p120RasGAP is a multidomain regulator of Ras signaling, containing two SH2 domains at its N-terminus and multiple other domains including a RasGAP. Binding of p190RhoGAP is mediated by phosphotyrosine-SH2 domain interactions, and a major driver is thought to be between the N-terminal SH2 of p120RasGAP and pTyr-1105 of p190RhoGAP. p190RhoGAP recruitment has multiple effects, including inhibition of Rho signaling by locating p190RhoGAP to the plasma membrane, and activation of Ras signaling by suppression of p120RasGAP’s RasGAP activity when it is bound to p190RhoGAP. Therefore, in this study we determine the crystal structures of the N-terminal SH2 domain of p120RasGAP alone, and its complex with a phosphorylated peptide corresponding to residues around and including pTyr-1105 of p190RhoGAP. The SH2 fold consists of a central β-sheet flanked by two α-helices, and both crystal structures reveal that the p120RasGAP N-terminal SH2 domain adopts this fold.

We next obtained co-crystals of the N-terminal SH2 domain of p120RasGAP in complex with a synthesized peptide, EEENI(p-Tyr)SVPHDST, corresponding to residues 1100 to 1112 of p190RhoGAP. The co-crystals diffracted to 1.6 Å resolution and contain one dimer per asymmetric unit. Good electron density is observed for all residues of the peptide except Thr-1112. The co-crystal structure reveals a broadly canonical interaction between p120RasGAP N-terminal SH2 domain and the p190RhoGAP pTyr-1105 peptide. The interaction buries 1290 Å2 of total surface area and the peptide binds perpendicular to the central SH2 domain β-sheet, with pTyr-1105 at position 0 and Pro-1108 at position +3 inserted into the expected pockets. pTyr-1105 is coordinated by a salt-bridge to Arg-207, which is the conserved arginine of the FLVR motif, also commonly referred to as ArgβB5 in SH2 convention. It is also coordinated by Arg-188 (ArgαA2) and Ser-209 (SerβB7). Interestingly, a three-residue cation-π stack is also observed between the phenyl-ring of pTyr-1105, Arg-231 and Arg-212. Pro-1108 of p190RhoGAP is inserted into the specificity determining SH2 hydrophobic pocket between βG and βE-βF loops. The pocket is defined by residues Phe-230, Leu-262, Ile-241 and Tyr-256. In the co-crystal structure, the βE-βF loop is stabilized by peptide binding which allows a hydrogen-bond to form between the carbonyl oxygen of Leu-262 and the backbone nitrogen of His-1109.

> GSTAPPTNQWYHGKLDRTIAEERLRQAGKSGSYLIRESDRRPGSFVLSFLSQMNVVNHFRIIAMSGDYYIGGRRFSSLSDLIGYYSHVSSLLKGEKLLYPVAPPEPVED;> XEEENIYSVPHDST[(4-{[4-(benzoylamino)phenyl]amino}-6-methoxyquinazolin-7-yl)oxy]acetic 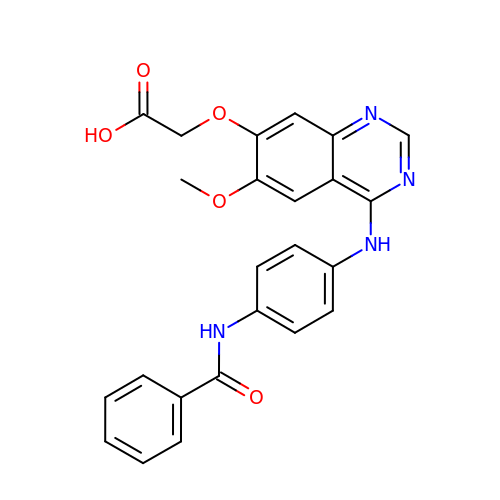acid | C24 H20 N4 O5 | VAJKCEBFUQHYLC-UHFFFAOYSA-N>[2x]GSMPMYEVQWKVVEESNGNNYSYIDPTQLPYDHKWEFPRNRLSFGKTLGAGAFGKVVEATAQGLIKSDAAMTVAVKMLKPSAHSTEREALMSELKVLSYLGNHENIVNLLGACTHGGPTLVITEYCCYGDLLNFLRRKRDEFVPYKVAPEDLYKDFLTLEHLLSFSYQVAKGMAFLASKNCIHRDLAARNILLTHGNITKICDFGLARDIKNDSNYVDKGNARLPVKWMAPESIFNSVYTFESDVWSYGIFLWELFSLGSSPYPGMPVDSKFYKMIKEGFRMSSPEYAPAEMYDIMKTCWDADPDKRPTFKQIVQDIEKQISESTNH

Avapritinib is the only potent and selective inhibitor approved for the treatment of D842V-mutant gastrointestinal stromal tumors (GIST), the most common primary mutation of the platelet-derived growth factor receptor α (PDGFRA). Against this background, we solve the crystal structures of avapritinib in complex with wild-type and mutant PDGFRA and stem cell factor receptor (KIT), which provide evidence and understanding of inhibitor binding and lead to the identification of a sub-pocket (Gα-pocket). Furthermore, we report the identification of a sub-pocket (Gα-pocket) located in the N-lobe of the kinase domain, which is surrounded by amino acids of key regulatory elements such as the Gly-rich loop and the αC-helix.

To our delight, we were able to obtain co-crystal structures at high resolutions for each of the inhibitors 8-12 bound to KIT-wt (1.5–2.0 Å) and 9 bound to PDGFRA-T674I (2.6 Å). A single modification by ethylation did not affect the potency significantly since the IC50 values were almost the same as for avapritinib. However, a reduction between 1.7- and 3.5-fold in potency was observed in the cellular experiments. A comparison of the obtained crystal structures indicated that the ethyl residue displaced one water molecule in the complex with KIT-wt. Yet, there were no other significant alterations in the complexes of KIT-wt and PDGFRA-T674I bound to 9 when compared to the complex structures bound to avapritinib, respectively. Lower inhibitory activity was observed in KIT cell lines for both alkylated derivatives 8 and 9 compared to PDGFRA cell lines.> 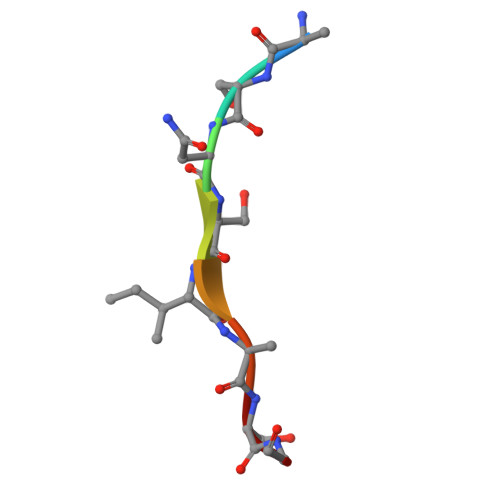ASNSIASG> MSLRRGIYHIENAGVPSAIDLKDGSSSDGTPIVGWQFTPDTINWHQLWLAEPIPNVADTFTLCNLFSGTYMDLYNGSSEAGTAVNGWQGTAFTTNPHQLWTIKKSSDGTSYKIQNYGSKTFVDLVNGDSSDGAKIAGWTGTWDEGNPHQKWYFNRMSVSSAEAQAAIARNPHIHGTYRGYILDGEYLVLPNATFTQIWKDSGLPGSKWREQIYDCDDFAIAMKAAVGKWGADSWKANGFAIFCGVMLGVNKAGDAAHAYNFTLTKDHADIVFFEPQNGGYLNDIGYDSYMAFY

The Marasmius oreades agglutinin (MOA) is the holotype of an emerging family of fungal chimerolectins and an active Ca2+/Mn2+-dependent protease, which exhibits a unique papain-like fold with special active site features. While acting as a dimerization domain, the papain-like domain of MOA retains the characteristic L-/R-domain partition of PLCPs. As additional feature, the MOA dimer carries two binuclear metal-binding clusters, symmetrically placed at the dimerization interface (Grahn et al., 2009). MOA requires the presence of calcium or manganese (II) to switch from the inactive form to an active protease (Cordara et al., 2011, Wohlschlager et al., 2011).

While other divalent cations cannot functionally replace calcium or manganese, cadmium or zinc inhibit the enzymatic activity of MOA (Cordara et al., 2011). Zinc and cadmium strongly inhibit the proteolytic activity of MOA and papain (Cordara et al., 2011, Shukor et al., 2006). It has been suggested that zinc binds at the catalytic center of PLCPs, directly coordinating the cysteine and histidine side chains of the catalytic dyad. To provide a structural basis for the inhibition, we collected anomalous diffraction data on MOA crystals grown in the presence of either zinc or cadmium. The anomalous difference maps of cadmium-containing crystals (calculated from data collected at 6.0 keV) show a similar feature, consistent with the previously suggested inhibition mechanism. Furthermore, zinc and cadmium inhibit the activity of MOA by forming a tight complex with the catalytic cysteine (Cys215) and histidine (His257), as predicted for papain. Finally, we showed in this work that complex formation of the catalytic dyad with metal ions like zinc or cadmium inactivates the enzyme.> PIEESLAAVIPISHLGEVGKWANNVLNCTEYSEKKIAERLYVFITFLTDMGVLEKINNLYKPANLKFQKALGLHDKQLTEETVSLTLNEYVLPTVSKYSDKIKSPESLYLLSSLRLLLNSLNALKLINEKSTHGKIDELTYIELSAAAFNGRHLKNIPRIPIFCILYNILTVMSENLKTESLFCGSNQYQYYWDLLVIVIAALETAVTKDEARLRVYKELIDSWIASVKSKSDIEITPFLNINLEFTDVLQLSRGHSITLLWDIFRKNYPTTSNSWLAFEKLINLSEKFDKVRLLQFSESYNSIKDLMDVFRLLNDDVLNNKLSEFNLLLSKLEDGINELELISNKFLNKRKHYFADEFDNLIRYTFSVDTAELIKELAPASSLATQKLTKLITNKYNYPPIFDVLWTEKNAKLTSFTSTIFSSQFLEDVVRKSNNLKSFSGNQIKQSISDAELLLSSTIKCSPNLLKSQMEYYKNMLLSWLRKVIDIHVGGDCLKLTLKELCSLIEEKTASETRVTFAEYIFPALDLAESSKSLEELGEAWITFGTGLLLLFVPDSPYDPAIHDYVLYDLFLKTKTFSQNLMKSWRNVRKV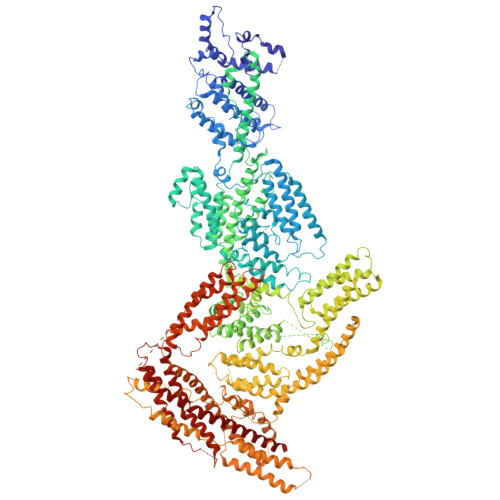ISGDEEIFTEKLINTISDDDAPQSPRVYRTGMSIDSLFDEWMAFLSSTMSSRQIKELVSSYKCNSDQSDRRLEMLQQNSAHFLNRLESGYSKFADLNDILAGYIYSINFGFDLLKLQKSKDRASFQISPLWSMDPINISCAENVLSAYHELSRFFKKGDMEDTSIEKVLMYFLTLFKFHKRDTNLLEIFEAALYTLYSRWSVRRFRQEQEENEKSNMFKFNDNSDDYEADFRKLFPDYEDTALVTNEKDISSPENLDDIYFKLADTYISVFDKDHDANFSSELKSGAIITTILSEDLKNTRIEELKSGSLSAVINTLDAETQSFKNTEVFGNIDFYHDFSIPEFQKAGDIIETVLKSVLKLLKQWPEHATLKELYRVSQEFLNYPIKTPLARQLQKIEQIYTYLAEWEKYASSEVSLNNTVKLITDLIVSWRKLELRTWKGLFNSEDAKTRKSIGKWWFYLYESIVISNFVSEKKETAPNATLLVSSLNLFFSKSTLGEFNARLDLVKAFYKHIQLIGLRSSKIAGLLHNTIKFYYQFKPLIDERITNGKKSLEKEIDDIILLASWKDVNVDALKQSSRKSHNNLYKIVRKYRDLLNGDAKTIIEAGLLYXXXXXXXXXXXXXXXXXXXXXXXXXXXXXXXRNIDTVASNMDSYLEKISSQEFPNFADLASDFYAEAERLRKETPNVYTKENKKRLAYLKTQKSKLLGDALKELRRIGLKVNFREDIQKVQSSTTTILANIAPFNNEYLNSSDAFFFKILDLLPKLRSAASNPSDDIPVAAIERGMALAQSLMFSLITVRHPLSEFTNDYCKINGMMLDLEHFTCLKGDIVHSSLKANVDNVRLFEKWLPSLLDYAAQTLSVISKYSATSEQQKILLDAKSTLSSFFVHFNSSRIFDSSFIESYSRFELFINELLKKLENAKETGNAFVFDIIIEWIKANKGGPIKKEQKRGPSVEDVEQAFRRTFTSIILSFQKVIGDGIESISETDDNWLSASFKKVMVNVKLLRSSVVSKNIETALSLLKDFDFTTTESIYVKSVISFTLPVITRYYNAMTVVLERSRIYYTNTSRGMYILSTILHSLAKN>GSHMRHRTLSSSPALWASIPCPRSELRLDLVLASGQSFRWKEQSPAHWSGVLADQVWTLTQTEDQLYCTVYRGDDSQVSRPTLEELETLHKYFQLDVSLAQLYSHWASVDSHFQRVAQKFQGVRLLRQDPTECLFSFICSSNNNIARITGMVERLCQAFGPRLIQLDDVTYHGFPNLHALAGPEAETHLRKLGLGYRARYVRASAKAILEEQGGPAWLQQLRVAPYEEAHKALCTLPGVGAKVADCICLMALDKPQAVPVDVHVWQIAHRDYGWHPKTSQAKGPSPLANKELGNFFRNLWGPYAGWAQAVLFSADLRQ[3x]

Our approach is applied to discover inhibitors of 8-oxoguanine DNA glycosylase (OGG1), an enzyme that is part of the DNA damage response pathway. OGG1 recognizes the presence of the oxidized nucleobase 7,8-dihydro-8-oxoguanine (8-oxoG) in DNA and initiates repair by excision of the damaged base. Recent studies demonstrate that inhibition of OGG1 is a promising strategy for the development of drugs against cancer and inflammation. The active site is highly polar and adopts different shapes in the complexes with the inhibitor and DNA, which are properties characteristic of challenging drug targets.

As commercial chemical space lacked elaborations of our most potent inhibitor, further optimization was driven by reaction-based enumeration of virtual libraries using commercial building blocks. Reagents compatible with Chan-Lam, Suzuki, Ullmann, or amide couplings were identified and reacted in silico to afford molecules with similar topologies as compound 7. The resulting synthetically accessible virtual library contained 6720 molecules that were not available in make-on-demand catalogs. As the docking was performed to the active site conformation of OGG1 observed in the complex with inhibitor 7, several compounds were designed to extend into the additional subpocket identified in this structure. In total, 16 compounds (8-23) were successfully synthesized in-house and detailed synthetic procedures are provided in the Supplementary Information. Twelve compounds showed comparable or better potencies than compound 7. Crystal structures of complexes were determined for two inhibitors (8 and 17). As the docking algorithm did not take protein flexibility into account, access to multiple structures of OGG1 representing different active site conformations was crucial for successful fragment elaboration.>[6x]MSEEIREVKVLEKPWVEKYRPQRLDDIVGQEHIVKRLKHYVKTGSMPHLLFAGPPGVGKTTAALALARELFGENWRHNFLELNASDERGINVIREKVKEFARTKPIGGASFKIIFLDEADALTQDAQQALRRTMEMFSS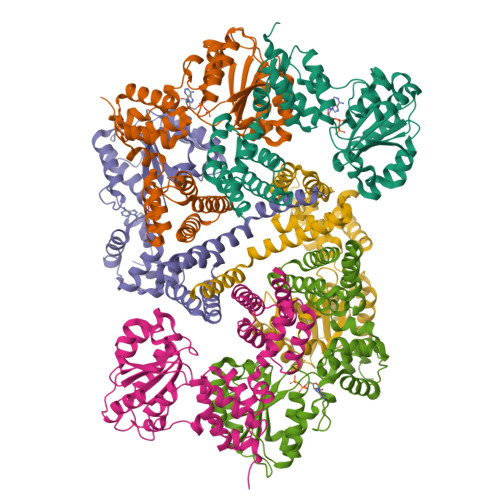NVRFILSCNYSSKIIEPIQSRCAIFRFRPLRDEDIAKRLRYIAENEGLELTEEGLQAILYIAEGDMRRAINILQAAAALDKKITDENVFMVASRARPEDIREMMLLALKGNFLKAREKLREILLKQGLSGEDVLVQMHKEVFNLPIEEPKKVLLADKIGEYNFRLVEGANEIIQLEALLAQFTLIGKK>PLFNDIAPGIPSITAYSKNGLKIEFTFERSNTNPSVTVITIQASNSTELDMTDFVFQADVPKTFQLQLLSP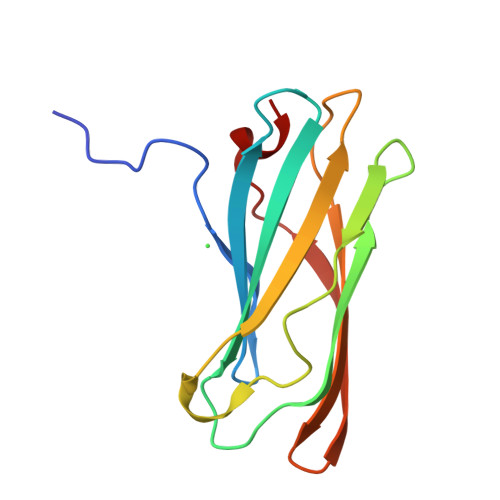SSSVVPAFNTGTITQVIKVLNPQKQQLRMRIKLTYNHKGSAMQDLAEVNNFPPQSWQ[2x]>[2x]MPKVILKGPLISQFNFREIYVNDRELLRVLVKIDSKKHLILNESNQLKSGILILINGKDWRLYRNQLLNDNDIIEIIPINHGGLEHHHHHH

The eukaryotic Urm1 (ubiquitin-related modifier-1) protein, which displays both structural and amino-acid sequence homology to the prokaryotic ThiS and MoaD, has been proposed as a candidate for the evolutionary ‘missing link' between the eukaryotic Ub/Ubl family and the ancestral prokaryotic sulphur-transfer proteins1617181920212223. Covalent attachment of the modifier, referred to as SAMPylation, occurs between the conserved C-terminal di-glycine motif of SAMP, and specific lysine residues on a variety of target proteins, in a manner reminiscent of urmylation and ubiquitylation. Here we solve the crystal structure of an Urm1/SAMP homologue from the related species S. solfataricus, which reveals similarities to both eukaryotic Urm1 proteins, and other archaeal SAMPs. Taken together, our data suggest that Urm1/SAMP modification acts as a signal for substrate recognition by the archaeal proteasome.

As predicted, the S. solfataricus Urm1 adopts a ubiquitin-like β-grasp fold, formed from a four-stranded β-sheet packed against a central α-helix. Similar to Ub and other Ubls, the β-strands are organized in the order β2-β1-β4-β3. Four α-helices are also evident, with the first connecting strands β1 and β2, the second and third located between strands β2 and β3, and the final helix positioned on a long loop between strands β3 and β4. Inspection of the surface hydrophobicity of the S. solfataricus Urm1 structure revealed the presence of a solvent-exposed hydrophobic patch in close proximity to the C-terminal tail. This surface is composed of the conserved hydrophobic residues L52 and L54 on strand β3, I77 on strand β4, and I79 on the C terminus of the protein. A second exposed hydrophobic surface is also present in S. solfataricus Urm1, formed by the residues I19 and V21 on strand β2, I33 at the end of helix α2, and F16, on the loop adjoining helix α1 and strand β2. We observed in the structure that a leucine (L67) on the final loop on one Urm1 subunit protrudes into the hydrophobic depression of a neighbouring Urm1 chain to form a dimerization interface. The structure also reveals a narrow hydrophobic channel, juxtaposed to the first hydrophobic patch abutting the C-terminal tail. This trough is lined with the surface exposed conserved residues L27, L47 and G50, and extends from the base of the C-terminal tail to the opposite end of the structure.>[4x]MNYPAEPFRIKSVETVSMISRDERVKKMQEAGYNTFLLNSKDIYIDLLTDSGTNAMSDKQWAGMMIGDEAYAGSENFYHLEKTVKELFGFKHIVPTHQGRGAENLLSQLAIKPGQYVAGNMYFTTTRFHQEKNGATFVDIVRDEAHDASLNLPFKGDIDLNKLATLIKEKGAEN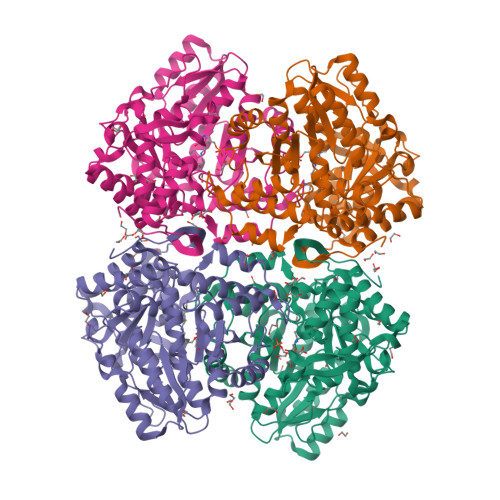IAYICLAVTVNLAGGQPVSMANMRAVHEMASTYGIKIFYDATRCVENAYFIKEQEAGYENVSIKDIVHEMFSYADGCTMSGKKDCLVNIGGFLCMNDEEMFSAAKELVVVYEGMPSYGGLAGRDMEAMAIGLREAMQYEYIEHRVKQVRYLGDKLREAGVPIVEPTGGHAVFLDARRFCPHLTQDQFPAQSLAASIYMETGVRSMERGIVSAGRSKETGENHRPKLETVRLTIPRRVYTYAHMDVVADGIIKLYQHKEDIRGLTFVYEPKQLRFFTARFDFI> MSLILVYSTFPNEEKALEIGRKLLEKRLIACFN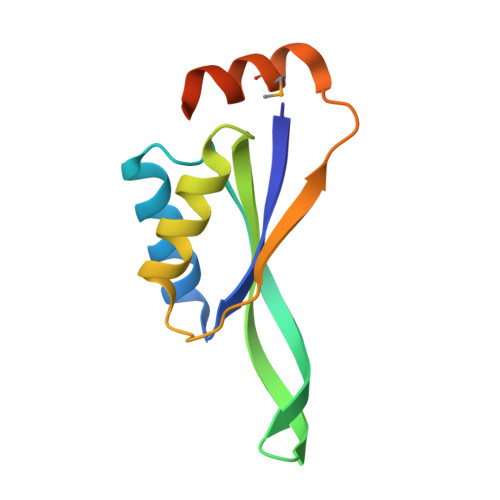AFEIRSGYWWKGEIVQDKEWAAIFKTTEEKEKELYEELRKLHPYETPAIFTLKVENVLTEYMNWLRESVLEGGSHHHHHH C. neoformans sterylglucosidase 1 (Sgl1), the first gene/protein identified with a sterylglucosidase activity, converts erg-glc to ergosterol and glucose. Our analysis of structures of C. neoformans Sgl1 reveals a Y-shaped hydrophobic active site pocket that generates specificity for erg-glc and which is not present in human and bacterial glucosylceramidases. Sgl1 is an ideal pharmacological target with broad spectrum since Sgl1 is widely conserved in fungi and there is no obvious homolog in humans.

Hit 1 is a piperidine derivative with good solubility (clogP 1.49) and an IC50 of 1 µM in our primary screen with res-glp as the substrate. To aid future medicinal chemistry optimization, we determined co-crystal structures of Hit 1 and Hit 9 with C. neoformans Sgl1 at 2.8 and 2.3 Å resolutions, respectively. Strong electron density for Hit 1 and Hit 9 was observed in all four Sgl1 molecules in the asymmetric unit, which allowed unambiguous modeling. Both compounds bound within the active site and formed a series of polar interactions near the catalytic site with the planar aromatic rings of the compounds occupying space in the buried hydrophobic pocket. The overall position of Hit 1 and Hit 9 were notably similar to the predicted docked erg-glc-binding pose. The piperidine ring of Hit 1 formed hydrogen bond interactions with the active site residues Glu270, Trp570, and Glu587, while the methyl-pyrrolidine ring of Hit 9 formed key interactions with Lys47, Glu270, and Glu587. Despite its lower potency in vitro and in cells, Hit 1 was chosen for animal experiments as it was predicted to have more optimal pharmacokinetic properties. In contrast, Hit 1 alone or in combination with fluconazole resulted in no CFU recovered from the brain.

>SMPPPPEVSPVTGNPVSPHYIHSSTLHFQDVNGRSLVLRGVNLSGSAKHPNNQPSHIREGFWETAEAGKGDFINKPLNLDDGSADLHLARLKAWGYNLLRYVFTWESLEHAGPKEYDYAYMDYIIAVLRKCKEWGFRVFMDPHQDVWSRFTGGSGAPLWTLYACGIDPYHLTATAAAYLHCEWPSAESPKPQDFPAMIWGTNYTHLANQTIWTFFFAGKTYAPKCIIDGKNIQDFLQDHFIDAVGELAKRIAEEAGDLLDECVIGWDSINEPGEGLIGCKDLAVIPAEQQLKKGPSPTPIEGMRLGMGEAQDVQAWNFGPMGPYRGSRQTIDPKGVKLWLSKEDDVKRGSGKWGWTRGKEWALGTCIWAHHGVWEIATSTLLRPDYFSTLPTNPGHQVDFVDDFWALHWLAYSSRIRLHHPESIHFIQAPVLRQPPKLPESFLKGRACSSPHFYDGLTLMTKHWNWFNADAIGVIRKKYWSIVQAVRIGEGPIRKMIQGELAVLKQDTIDILGNYPTLVGEIGIPYDMDDKKAYGYVDGGRGEGDYSSQQKAMDCSMNACDGPNCLNYAIWNYVPDNVHEWGDNWNGEDLSLWSVDDKEQESYHDSPRSDTPNFSTNSNSLTNSSATLTVPMSGASKLRPSPSVIDSGDFSPTLILDGSRAVAAFCRPYPVATVGIPERIDFDITSTKFKYAVRVRADDIANEQVYTEIYLPFVHYAASLNASYSSFAQLSLDVTIVASHGRVEIQGQTLRWWYPVPGTGEEVYTIEVQRNGGALRRDLGYVQQGNFLDVCPECVIA[4x]> SVRSSSRTPSDKPVAHVVANPQAEGQLQWLNRRANALLANGVELRDNQLVVPSEGLYLIYSQVLFKGQGCPSTHVLLTHTISRIAVSYQTKVNLLSAIKSPCQRETPEGAEAKPWYEPI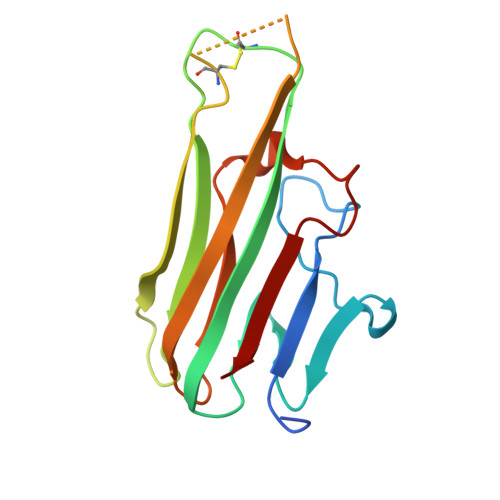YLGGVFQLEKGDRLSAEINRPDYLDFAESGQVYFGIIAL> CQPIFLNVLEAIEPGVVCAGHDNNQPDSFAALLSSLNELGERQLVHVVKWAKALPGFRNLHVDDQMAVIQYSWMGLMVFAMGWRSFTNVNSRMLYFAPDLVFNEYRMHKSRMYSQCVRMRHLSQEFGWLQITPQEFLCMKA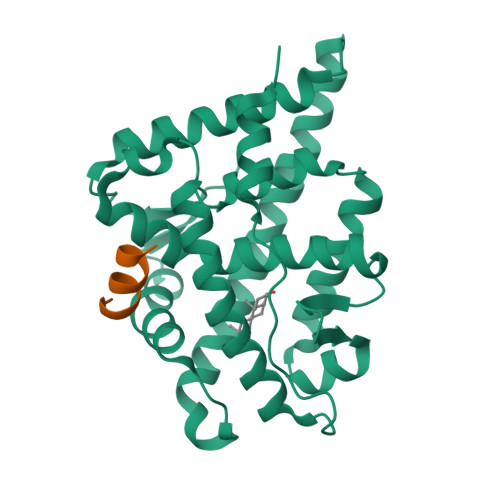LLLFSIIPVDGLKNQKFFDELRMNYIKELDRIIACKRKNPTSCSRRFYQLTKLLDSVQPIARELHQFTFDLLIKSHMVSVDFPEMMAEIISVQVPKILSGKVKPIYFHTQ;> RETSEKFKLLFQSYN>MSHQIRSKKTLWELVGRNKDALRDFLKEHRGTILLRDIASEHKVVYKPIFKRYNGDPDLIEDNSND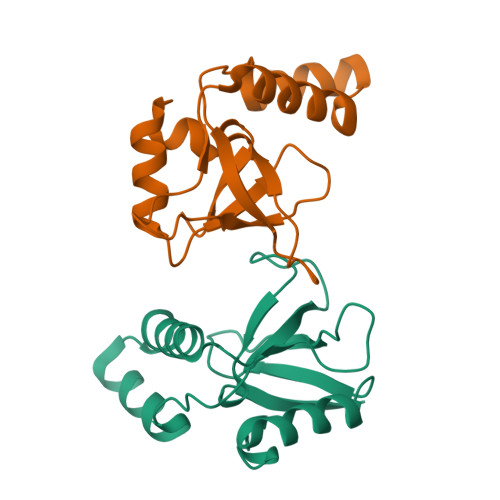VEHWYDYHLERYWNTPELKKEFYKKFGPVDLNQPIILAKPLRQHNRGDLVHLLPQFVVPVYN[2x]> MTEFVNRG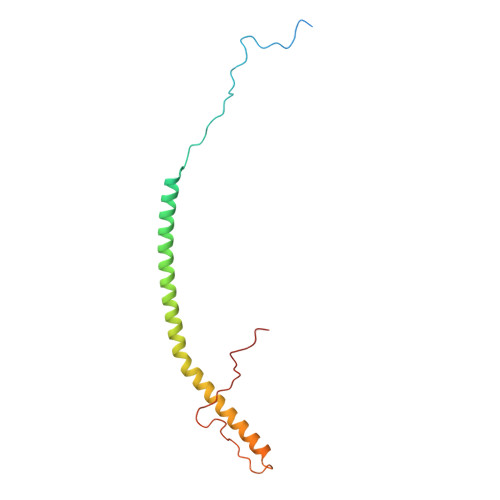FPGLKSIKDLPKVQDVPPPGGFPSIRIERKLPNTGPTGLAVFLGFTAFMALAVNQARDRKSTNRLEAEEVYTARSILHPILQAEWDLRYLEHQRKEREDEAKIMKDVPGWKVGEATSRRRWLPPVESFDVRPLI> UGCUCCUAGUACGAGAGGACCGGXGUG

Deazapurine nucleosides such as 3-deazaadenosine (c3A) are crucial for atomic mutagenesis studies of functional RNAs. The replacement of a single nitrogen atom by a carbon atom can be critical because the acid-base properties of the nucleobase are dramatically changed and hydrogen acceptor/donor properties are erased at the specific position (6–8). We utilized the 27 nt fragment of the E. coli 23S rRNA sarcin−ricin loop (SRL) which is a robust and well-behaved crystallization scaffold.

Oligoribonucleotides of 27 nucleotide length corresponding to the sequence of Escherichia coli 23 S rRNA sarcin-ricin loop (SRL) and containing a 3-deazaadenosine at position 2670 were used for crystallization. For the incorporation of c3A, we deemed nucleotide A2670 appropriate, which forms a Watson−Crick base pair with C2650 in the regular A-form double helical region. X-ray structure determination showed that the c3A nucleobase is well-defined in the electron density maps for the c3A-modified RNA. Superimpositions of the c3A-modified RNA structure with the unmodified RNA showed a root-mean-square deviation (rmsd) of 0.12 Å (within the errors on coordinates of 0.13 Å). Overall, the structure revealed that the 3-deazanucleobase does not significantly affect the base pair geometry and the SRL RNA fold. However, what is different is the local hydration network in the minor groove of the c3A–U base pair. While three ordered water molecules are found in the minor groove for the unmodified base pair, four are observed for the modified base pair. An obvious distinction is that the N3 atom of A2670 is hydrogen-bonded to one of the water molecules (2.8 Å distance) while for the c3A2670/U2650 base pair, a continuous hydrogen-bonded water chain spans from the 2′-OH of c3A2670 to the 2′-OH of U2650 without involving the c3A nucleobase; the closest water is in 3.3 Å-distance from its C3 atom. Although these structural differences in the hydration pattern appear minor in the static X-ray structure, they may contribute to increased base pair opening dynamics as reflected in the imino proton NMR spectrum of the c3A modified SRL RNA by significant signal broadening. The structure points out that the hydrophobic minor grove face of c3A impairs hydration because the water molecule that is usually hydrogen bonded to the N3 atom becomes extruded from the 3-deaza-modified base pair.>SVRRDRAPPERGGAGTSQDGTSKNWFKITIPYGRKYDKAWLLSMIQSKCSVPFTPIEFHYENTRAQFFVEDASTASALKAVNYKILDRENRRISIIINSSAPPHTILNELKPEQVEQLKLIMSKRYDGSQQALDLKGLRSDPDLVAQNIDVVLNRRSCMAATLRIIEENIPELLSLNLSNNRLYRLDDMSSIVQKAPNLKILNLSGNELKSERELDKIKGLKLEELWLDGNSLCDTFRDQSTYISAIRERFPKLLRLDGHELPPPIAFDVEAPTTLPPCKGSYFGTENLKSLVLHFLQQYYAIYDSGDRQGLLDAYHDGACCSLSIPFIPQNPARSSLAEYFKDSRNVKKLKDPTLRFRLLKHTRLNVVAFLNELPKTQHDVNSFVVDISAQTSTLLCFSVNGVFKEVDGKSRDSLRAFTRTFIAVPASNSGLCIVNDELFVRNASSEEIQRAFAMPAPTP[2x];>ASVDFKTYVDQACRAAEEFVNVYYTTMDKRRRLLSRLYMGTATLVWNGNAVSGQESLSEFFEMLPSSEFQISVVDCQPVHDEATPSQTTVLVVICGSVKFEGNKQRDFNQNFILTAQASPSNTVWKIASDCFRFQDWAS[2x]

The movement of transcripts through NPCs is mediated by NXF1:NXT1 (also known as TAP:p15), which is the metazoan homolog of Mex67:Mtr2, the principal mRNA export factor in Saccharomyces cerevisiae. NXF1 is a modular protein comprised of four domains: an N-terminal RNA recognition motif (RRM), a leucine-rich repeat (LRR), a nuclear transport factor 2-like domain (NTF2L) and an ubiquitin-associated (UBA) domain. NXT1/p15 is a 15-kDa protein that also has an NTF2-like fold and which forms a heterodimer with NXF1 via the NTF2L domain. To do this, type-D retroviruses have a ∼130 nucleotide long RNA element known as the constitutive transport element (CTE) in the 3′ end of their single-stranded RNA genome that binds to NXF1:NXT1 without the need for adapter proteins.

We present here the crystal structure of the complex formed between Homo sapiens NXF1 from which the N-terminal 95 residues and the UBA domain had been removed (NXF1ΔNΔUBA) and NXT1 and show that it has a novel homodimeric domain-swapped configuration generated by a interaction between the linker between the LRR and NTF2L domains with NXT1. Because the linker between the C-terminal UBA domain and the remainder of NXF1 is thought to be very flexible and the N-terminal 95 residues of NXF1 are thought to have an auto-inhibitory role in mRNA binding, these two regions were deleted to facilitate crystallization and analysis of RNA binding. The asymmetric unit contained two copies of the complex that were arranged to form a domain-swapped dimer. Density for the RRM domain was not observed, probably as a result of its not having a well-defined position as a consequence of the flexibility of the RRM–LRR linker. Strikingly, the position of the LRR domain relative to the NTF2L:NXT1 region was the same in both copies. In addition to the interaction between the pre-α1 loop with the canonical NXT1 copy, the linker between the LRR and NTF2L domain also made contacts with the alternate non-canonical copy of NXT1 in a domain swapped manner (blue on orange). Hydrophobic contacts also dominated this interaction interface, where Ile360, Phe362 and Val364 were buried in a cavity of the non-canonical copy of NXT1. The resultant domain-swapped dimer generates a flat platform with 2-fold symmetry in which the three pairs of RNA-binding domains (RRM, LRR and NTF2L domains) are all arranged on one face that results in their being ideally placed to interact with a dimeric binding motif such as that found in the CTE. Consistent with the requirement that the nucleoporin binding sites of NXF1:NXT1 need to be available while mRNA cargo is bound, the putative nucleoporin binding sites consisting of the residues 486–491 and 519–521 and 527 of NXF1 were found on the opposite face of the NTF2L:NXT1 dimer.>[4x]MNHKVHHHHHHIEGRHMTPSISKDAPIKGSITISKKGATFTAYKLLDATKSGDAYEYSVNSDLKDFFNNSNYGSYSQESIQKLSGEEVKEFAVKLHKYVLDNKKSGKELTDGQKNTVDLGYYLVTEASSDSEGAAVASTPIIVSVPQVSGDSWNYDVTINPKDNTPILEKNIVKENQRVKTSSENIGDVVKYEVKASIPVYQKNAQDIMYKFTDTM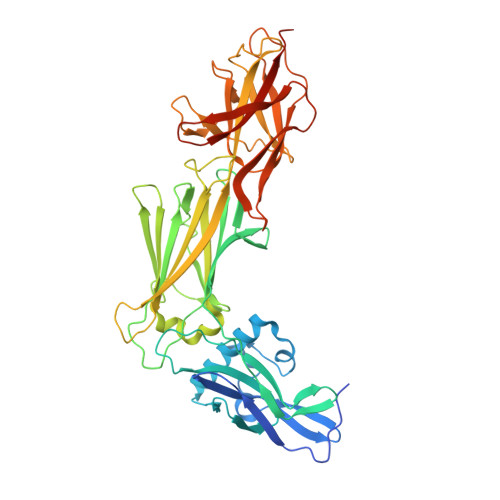SKGLTYDEKTGFKVTSGDKVFAKDKDYTVEVKKQEDGETVITINFVYENIKAYAETGITLNYQATLNKDVVISNKENLGNTNNIQLDYTNNPHVKDSYKKLTDKVTTYTFGFGITKVDSELNSKLLQGAEFSVKDESGKTVAKYTYDEKGQVVSLSGNGVTNSKGITTFVGLKEGKYLITEEVAPSGYSLLKNPVEVTITANKDESGKYTGAATIEISNGNKAGQIINDISENDGNILFNVQIENHAGFSLPSTGGLGNT1-{1-[(2-methyl-1,3-thiazol-4-yl)methyl]piperidin-4-yl}methanamine | C11 H19 N3 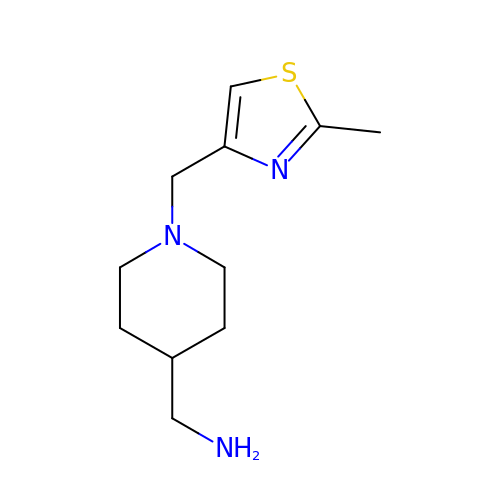S | ZEYZIFKDRCDRKU-UHFFFAOYSA-N>[4x]MGSDKIHHHHHHMKIDILDKGFVELVDVMGNDLSAVRAARVSFDMGLKDEERDRHLIEYLMKHGHETPFEHIVFTFHVKAPIFVARQWFRHRIASYNELAGRYSKLSYEFYIPSPE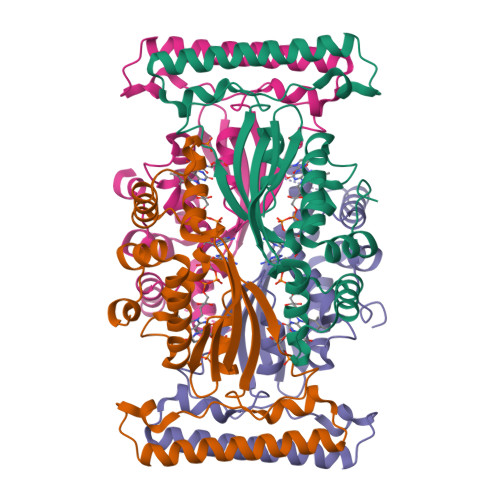RLEGYKTTIPPERVTEKISEIVDKAYRTYLELIESGVPREVARIVLPLNLYTRFFWTVNARSLMNFLNLRADSHAQWEIQQYALAIARIFKEKCPWTFEAFLKYAYKGDILKEVQV>[5x]GMEVLDLVTGPDSVTEIEAFLNPRMGQPPTPESLTEGGQYYGWSRGINLATSDTEDSPENNTLPTWSMAKLQLPMLNEDLTCDTLQMWEAVSVKTEVVGSGSLLDVHGFNKPTDTVNTKGISTPVEGSQYHVFAVGGEPLDLQGLVTDARTKYKEEGVVTIKTITKKDMVNKDQVLNPISKAKLDKDGMYPVEIWHPDPAKNENTRYFGNYTGGTTTPPVLQFTNTLTTVLLDENGVGPLCKGEGLYLSCVDIMGWRVTRNYDVHHWRGLPRYFKITLRKRWVK

Murine Polyomavirus (MuPyV) is a double-stranded DNA virus that can induce tumors in newborn animals. Viral attachment is mediated by the major capsid protein, VP1, which forms pentameric capsomers that assemble into the T = 7d icosahedral capsid of the virus. Sialylated oligosaccharide receptors are engaged in a shallow groove on top of VP1 formed by loop structures on the protein surface, similar to other polyomaviruses. The differences among the three strains have been mapped to amino acid variations at two positions, 91 and 296, within the receptor-binding region of VP1.

The human milk hexasaccharide DSLNT is the glycan portion of the lacto-series ganglioside 3’-6’-isoLD1, which is overexpressed in the central nervous system. In contrast to GT1a and GD1a, DSLNT does not contain an [α-2,3]-linked Neu5Acd as a short arm but instead a branching [α-2,6]-linked Neu5Acc. While PTA and LID do bind DSLNT, the complex structures do not show any electron density for the Neu5Acc, indicating that this sugar is conformationally flexible and does not contribute contacts. When bound to the PTA strain, the stem of DSLNT is moderately rearranged. In comparison to GalNAc in GT1a, the GlcNAc moiety is slightly tilted away from E91 due to a ~20° rotation of the psi angle in the Gala-[β-1,3]-GlcNAc linkage (assessed using CARP) that propagates throughout the sugar. In addition, there is no visible electron density for the GlcNAc O6 that is engaged in the [α-2,6]-branching as well as an increased B-Factor variance within the glycan. The reason for the sideward twist and the missing electron density for Neu5Acc observed in PTA is probably the electrostatic repulsion between the carboxyl groups of Neu5Acc and E91. While the charge of E91 is compensated by K186, as was hypothesized before, the two carboxylate groups would come within about 2 Å of one another if DSLNT bound to PTA in the same way as observed in RA. This hypothesis is confirmed by a PTA E91Q mutant that rescued binding of Neu5Acc. The DSLNT glycan binds similarly to all three strains, with the lowest overall affinity.> MMWKIAVVDDDKNILKKVSEKLQQLGRVKTFLTGEDFLNDEEAFH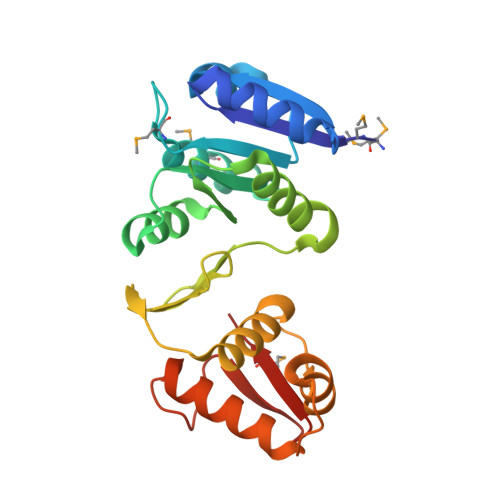VVVLDVMLPDYSGYEICRMIKETRPETWVILLTLLSDDESVLKGFEAGADDYVTKPFNPEILLARVKRFLEREKKGLYDFGDLKIDATGFTVFLKGKRIHLPKKEFEILLFLAENAGKVVTREKLLETFWEDPVSPRVVDTVIKRIRKAIEDDPNRPRYIKTIWGVGYMFTGGER> MSESQTLDKVYQMKSKPRGYCLIINNHNFAKAREKVPKLHSIRDRNGTHLDAGALTTTFEELHFEIKPHDDCTVEQIYEILKIYQLMDHSNMDCFICCILSHGDKGIIYGTDGQEAPIYELTSQFTGLKCPSLAGKPKVFFIQACQGDNYQKGIPVETDSEEQPYLEMDLSSPQTRYIPDEADFLLGMATVNNCVSYRNPAEGTWYIQSLCQSLRERCPRGDDILTILTEVNYEVSNKDDKKNMGK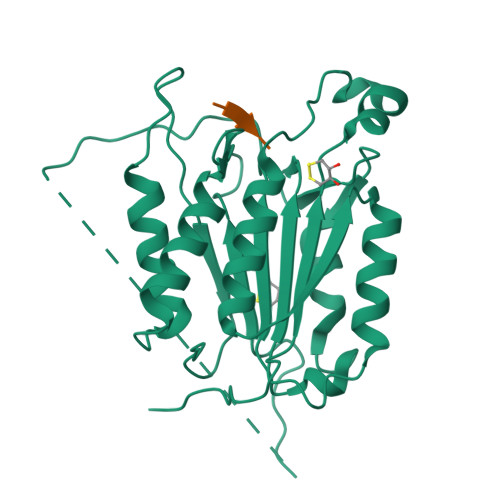QMPQPTFTLRKKLVFPSDAAALEHHHHHH 tert-butyl 4-[3-amino-6-(2-hydroxyphenyl)pyridazin-4-yl]piperazine-1-carboxylate 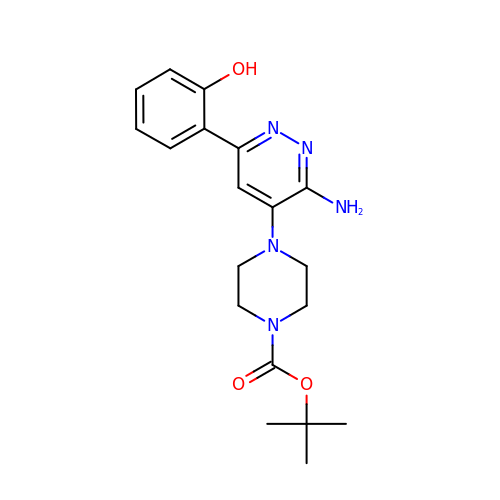| C19 H25 N5 O3 | AQTNUGRRZDRZIA-UHFFFAOYSA-N> SLEARAALNQALEMKRQGKREKAQKLFMHALKMDPDFVDALTEFGIFSEEDKDIIQADYLYTRALTISPYHEKALVNRDRTLPLVEEIDQRYFSIIDSKVKKVMSIPKGNSALRRVMEETYYHHIYHTVAIEGNTLTLSEIRHILETRYAVPGKSDEEQNEVI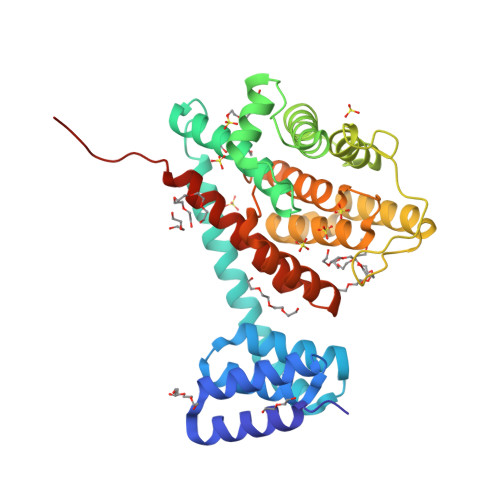GMHAAMKYINTTLVSRIGSVTISDVLEIHRRVLGYVDPVEAGRFRTTQVLVGHHIPPHPQDVEKQMQEFVQWLNSEEAMNLHPVEFAALAHYKLVYIHPFIDGNGRTSRLLMNLILMQAGYPPITIRKEQRSDYYHVLEAANEGDVRPFIRFIAKCTETTLDTLLFATTEYSVALPEAQP> PVFAKA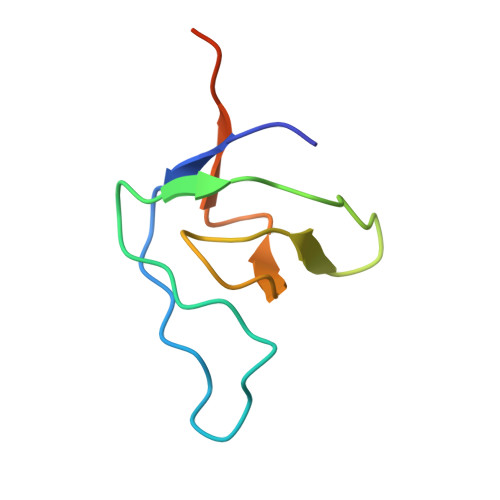IQKRVPCAYDKTALALEVGDIVKVTRMNINGQWEGEVNGRKGLFPFTHVKIFDPQNPDENE>MSENERPGLLGRVMSAFKPKAADAVTVASFSQRDAGLYIGSRFTSDAGREVSVQTAMSLDAVQACVKLISQSIAAMPLYLYKKTPDGRKEAVNHPLYDLLLSAPNSSQTAFEFFECILTAMLLHGNAYVRKLMSNGKIESLQFMHSSRLTISQDARGAYKYAYRKLDGTQIDVPSAQVWKIRGYSLDGENGISAIQYGAQVFGTALAAERQAGRAFTNGNLQQIYYSVAAFLTPEQREQFSANVAQSVESGRTPVLEGGIDVKALGLNPADAQLLQSRNYSVESICRFFAVPPSMIGHASAGTTSWGSGIEAQQLAFLGLTLAPWLRRIEQSLSLDLLTPGERRQYFVDYDVTTLLRADSAARSSFYATMVNNGVMTRDECREAEGLPKLGGNASVLTVQSAMVPLDEITNNTGADPAAAQGTTSLDRSAQ[2x];>[2x]MALTLAMVQRHLQADLIEDDERSYVMEQLLPAARESAEMFLNRNIYSTSEELAAAVAAGTAGQYPLVTPRAVEQAILLMLGDFYRDREATGKPVSTSAHNLLYPYRVKVGV;> MPISAGSLKTRLLAQRRTSGTDDWGAPVQGWSDLGLFSGDVKNDTGLGAIRTAAGSGLPASIAKYSIKVRSEVIRRWSINSADRIIGRLPFSTQEMVFSVTGVISDFADPSMAYILVEAGADEQ;> MTYGPILKQLLSPYFSGRVFPDAAPDVPGQDPYVIYQRVGGIPTYFTEGALADKANARVQLEVWSTSKQATYEAMVHIMRSVAAAPAMEPLGQPIDDYEPALRIYGSRVDISMYYNLT;>MALTLPKGIVFGFAPITSTTSSVTGVTRAAPPVATGTMLTAGTTVLVRSNTWTGINNRISVVDANKALQGFDTTDTTTYPGTSGP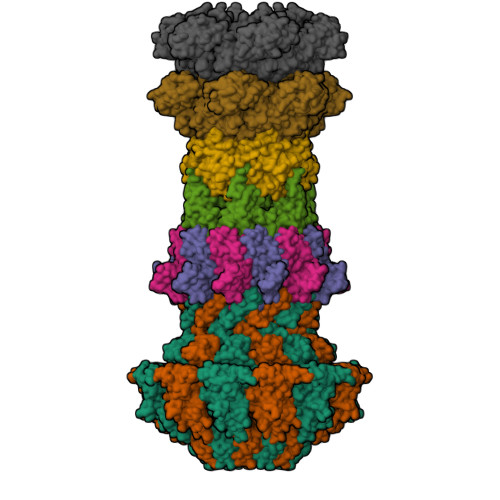VELITVGAFVNFTQQGEPSTSGGDQQFWNGQLLEDRSGRQLAIPTFKNAKTLTLPLYMDTSLPWYAAAKAADARGEPVAVRMLLPNGDASYNYGYMSFDGDATITANAPITNVATFTFLSDSTLVEA[2x]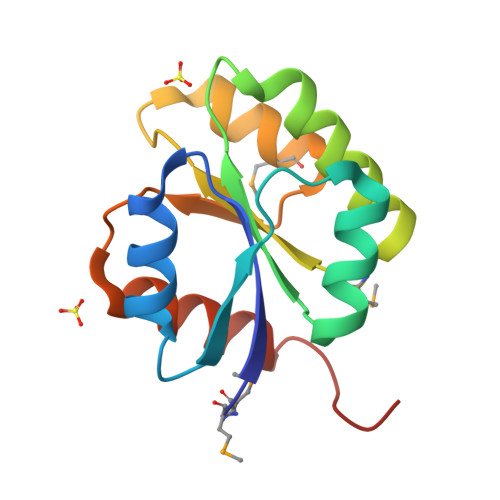>[8x]GMNQNFVALTQHPGELDWLQNSLASAGQVVPAGSASLEELLALLDVTAAGVLFISLGKSNLVSQGALVEGLVSARPMLSVVAIGDGLDNQLVLAAMRAGARDFITYGARASELTGLIRRLGGRLPSVPVSA>UNNGAC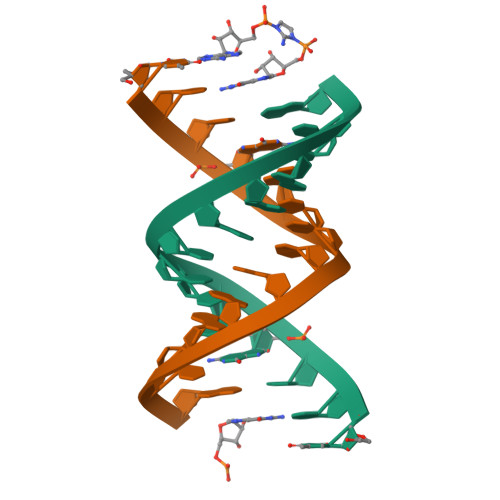UUAAGUCG[4x]>MSNDHPQPLDAAEIPRFAGIPTFMRLPAFTDPAALQVGLIGVPWDGGTTNRAGARHGPREVRNLSSLMRKVHHVSRIAPYDLVRVGDLGDAPVNPIDLLDSLRRIEGFYRQVHAAGTLPLSVGGDHLVTLPIFRALGRERPLGMVHFDAHSDTNDRYFGDNPYTHGTPFRRAIEEGLLDPLRTVQIGIRGSVYSPDDDAFARECGIRVIHMEEFVELGVEATLAEARRVVGAGPTYVSFDVDVLDPAFAPGTGTPEI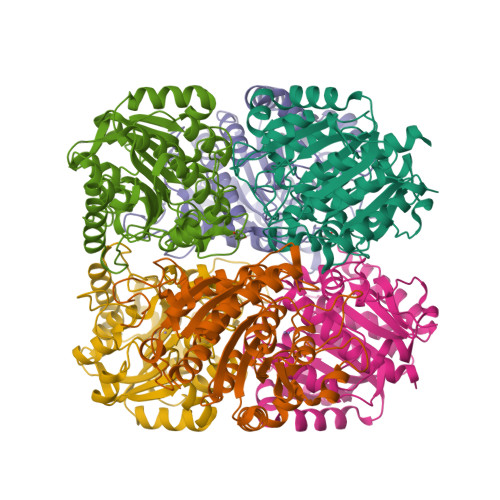GGMTSLQAQQLVRGLRGLDLVGADVVEVSPPFDVGGATALVGATMMFELLCLLAESAARSALEHHHHHH[2x]>[2x]DKMTIEVPVLTFVPVQVSAELENRGCWVKFFDKKNF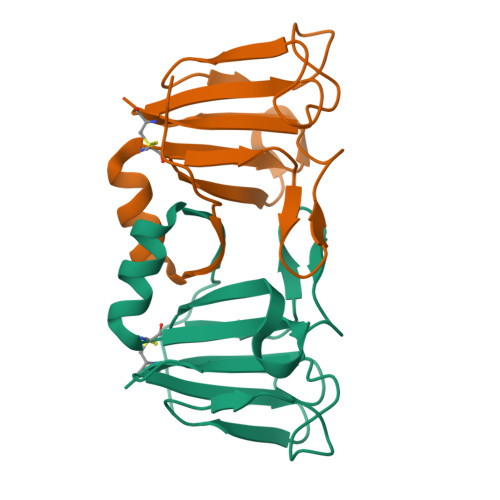QGDSLFLSGPATLPRLIGPFGYDWENKVRSVKVGPRANLTIFDNHNYRDEDKFLDAGANVANLSKEMGFFDNFRSMVLNCI>[2x]GPGSRYPVRRLPFSTVSKQDLAAFERIVPGGVVTDPEALQAPNVDWLRTLRGCSKVLLRPRTSEEVSHILRHCHERNLAVNPQGGNTGMVGGSVPVFDEIILSTARMNRVLSFHSVSGILVCQAGCVLEELSRYVEERDFIMPLDLGAKGSCHIGGNVATNAGGLRFLRYGSLHGTVLGLEVVLADGTVLDCLTSLRKDNTGYDLKQL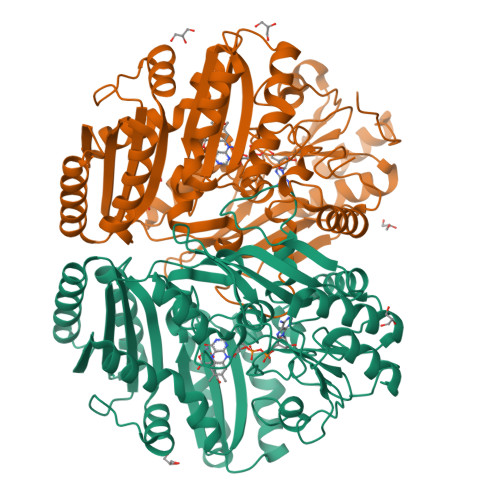FIGSEGTLGIITTVSILCPPKPRAVNVAFLGCPGFAEVLQTFSTCKGMLGEILSAFEFMDAVCMQLVGRHLHLASPVQESPFYVLIETSGSNAGHDAEKLGHFLEHALGSGLVTDGTMATDQRKVKMLWALRERITEALSRDGYVYKYDLSLPVERLYDIVTDLRARLGPHAKHVVGYGHLGDGNLHLNVTAEAFSPSLLAALEPHVYEWTAGQQGSVSAEHGVGFRKRDVLGYSKPPGALQLMQQLKALLDPKGILNPYKTLPSQAHHHHHH> MKRQGKRPSKNLKARCSRKALHVNFKDMGWDDWIIAPLEYEAFHCEGLCEFPLRSHLEPTNHAVIQTLMNSMDPESTPPTCCVPTRLSPISILFIDSANNVVYKQYEDMVVESCGCR;> ETGQCRIQKCTTDFVSLTSHLNSAVDGFDSEFCKALRAYAGCTQRTSKACRGNLVYHSAVLGISDLMSQRNCSKDGPTSSTNPEVTHGTKH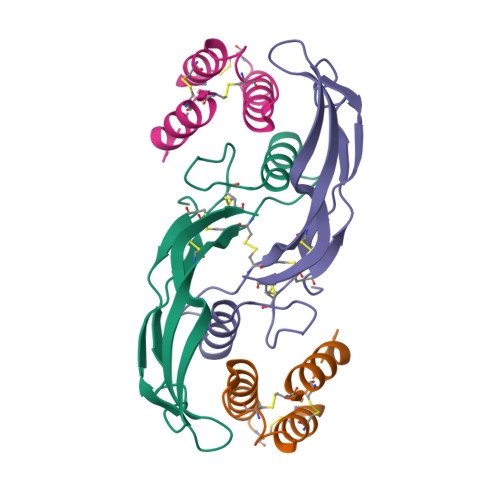HHHHH> AASCVLLHTGQKMPLIGLGTWKSEPGQVKAAIKYALTVGYRHIDCAAIYGNELEIGEALTETVGPGKAVPREELFVTSKLWNTKHHPEDVEPALRKTLADLQLEYLDLYLMHWPYAFERGDNPFPKNADGTIRYDATHYKDTWKALEALVAKGLVRALGLSNFSSRQIDDVLSVASVRPAVLQVECHPYLAQNELIAHCQARGLEVTAYSPLGSSDRAWRDPNEPVLLEEPVVQALAEKYNRSP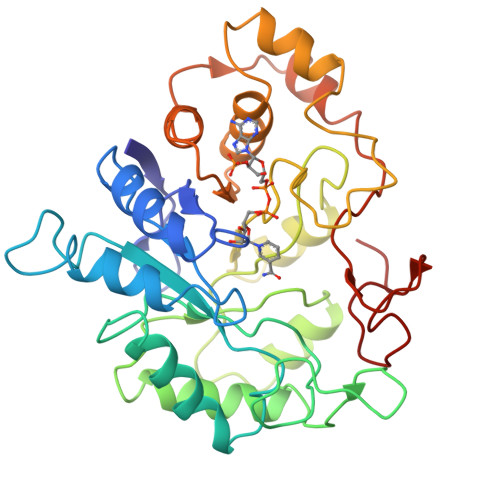AQILLRWQVQRKVICIPKSVTPSRIPQNIQVFDFTFSPEEMKQLDALNKNLRFIVPMLTVDGKRVPRDAGHPLYPFNDPY> MASLTAACRISARMAGRSVRGFRTSAAALAAQNFTMPALSPTMTEGNIATWRVKEGDKFSAGDVLLEIETDKATMDVEAQDDGVMVKIMKNDGAKGVAVGARIAVIAEEGDDISSLEIPADAAPQSKPAESAPSAPPPPTTADQSNVAVPESAPQNASSKSAPKPPKRQYPHYPSVAHLLKVNGIDAAAVKDITPTGPGGRLLKGDVLAYLGKINAQTPSTVSERFEKQSHLDLSNIKVAKS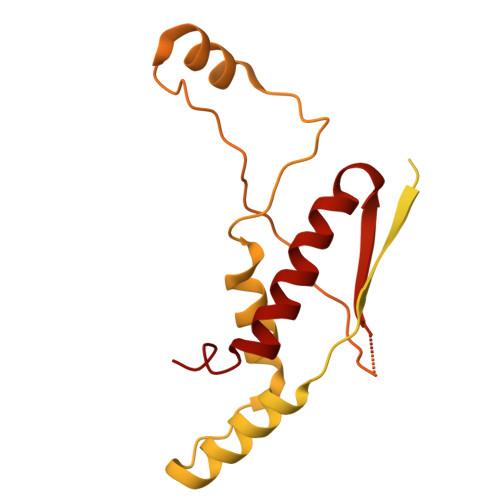TEAVKATTEKAQSKKLDAPAPPPVAVVTAPISLSAAIDVQNKLHKTIGVFLPLSTFITRATEIANQKLPLPANYQPTADELFNQVLGLDKVTRKESRGSYTPTFGSFVAPQRAARKADIIDILAAPSTRVAASAQSKSAAPGLTTSGPNVFSLQVPKSEEKRAQAFLQKMKLVLEQEPDKLVRA4-[(furan-2-yl)methyl]-1lambda~6~,4-thiazinane-1,1-dione | C9 H13 N O3 S 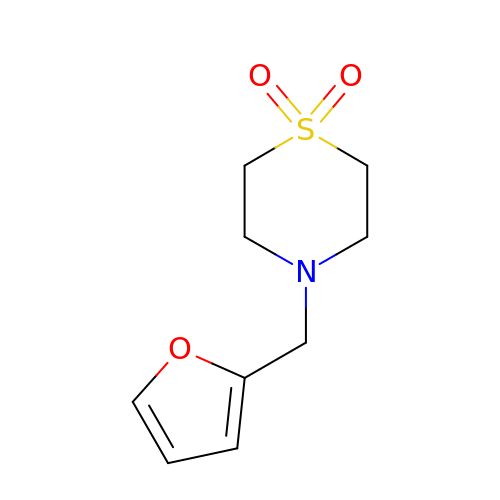| AEOGPIJVSQTAII-UHFFFAOYSA-N> GTVAL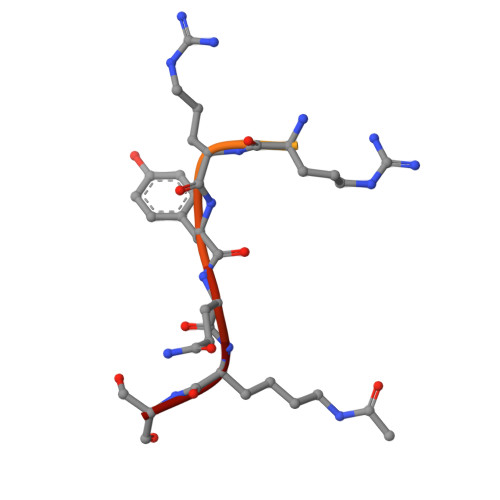REIRRYQKS>[2x]MKSVITTVISAADSAGRFPSSSDLESVQGNIQRASARLEAAEKLASNHEAVVKEAGDACFGKYGYLKNPGEAGENQEKINKCYRDIDHYMRLVNYSLVIGGTGPLDEWGIAGAREVYRTLNLPTSAYIAAFAFTRDRLCGPRDMSAQAGVEYSTALDYIINSLS;>[2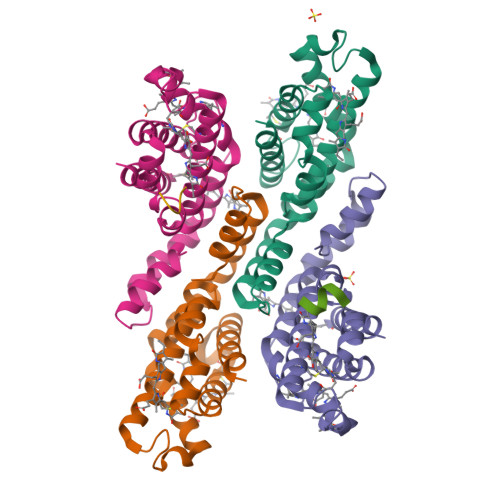x]MLDAFSRVISNADAKAAYVGGSDLQALRTFISDGNKRLDAVNYIVSNSSCIVSDAISGMICENPGLITPGGNCYTNRRMAACLRDGEIILRYISYALLAGDSSVLEDRCLNGLKETYIALGVPTNSTVRAVSIMKAAVGAFISNTASQRKGEVIEGDCSALAAEIASYCDRISAAVS;>AAFRAA[2x]In non-spherical bacteria, the actin homologue MreB is essential for shape maintenance as depletion of MreB through genetic knockouts or MreB-targeted drug treatment results in misshapen cells that eventually lyse. The MreB fibres are attached to the cell membrane via a hydrophobic loop in Thermotoga maritima as well as Gram+ bacteria and via an additional N-terminal amphipathic helix in Gram− bacteria. Here, we demonstrate that MreB from Caulobacter crescentus forms pairs of antiparallel protofilaments as revealed by crystal structures, an architecture unprecedented among actin-like proteins. The crystal structure of Caulobacter MreB (ΔCcMreBdh) reveals the typical actin fold, containing two domains on either side of a nucleotide binding cleft (Kabsch and Holmes, 1995).

Crystal structures of CcMreB in different nucleotide states, either as a monomer or as a polymer, were determined to a resolution better than 2 Å. Most crystal structures were obtained using ΔCcMreBdh, which behaved biochemically better than the full-length protein, yet was still showing correct filament formation as presented in Figure 6—figure supplement. It revealed that ΔCcMreBdh has the highest affinity for ATP (Kd ∼1 µM), followed by ADP (Kd ∼4 µM) and ATPγS (Kd ∼4.6 µM) and finally by AMPPNP (Kd ∼65 µM). Once MreB is in the polymeric state, the presence or absence of nucleotide has very little effect on the overall structure, which is presumably stabilised by inter- and intra-protofilament contacts. From the ΔCcMreBdh co-crystal structures with ADP and AMPPNP, it is clear that the active site could well accommodate a guanidine instead of an adenine as the major contacts are with the ribose and phosphate moieties of the nucleotide, a feature, again, shared with ParM.

> MISNDIAIDLGTANTLIYQKGKGIVLNEPSVVALRNVGGRKVVHAVGIEAKQMLGRTPGHMEAIRPMRDGVIADFEVAEEMIKYFIRKVHNRKGSGNPKVIVCVPSGATAVERRAINDSCLNAGARRVGLIDEPMAAAIGAGLPIHEPTGSMVVDIGGGTTEVAVLSLSGIVYSRSVRVGGDKMDEAIISYMRRHHNLLIGETTAERIKKEIGTARAPADGEGLSIDVKGRDLMQGVPREVRISEKQAADALAEPVGQIVEAVKVALEATPPELASDIADKGIMLTGGGALLRGLDAEIRDHTGLPVTVADDPLSCVALGCGKVLEHPKWMKGVLESTLAGSHHHHHH>SNAASATETNTAPSADTQAPKPVNTVTSDVDCSVSAAWGLYKFNQKSNFSAEFEMPESVKAGTGFDALIKIKDISVSNDNLSGYKNAKLTKSSIRINVGKNVKLDGNQPGLSLSNGVLSINDHLKASLEGNSLRISAAPITVRLQALTEGTLTFIPEKTILTNTASVDGYTANTTCTTNADKPFATVKVDPADGLTITAPESASIKQDVQITATVPEKLNEKMDGKVQFFVNHIAAGDPVPVTEDNKASTSIIFDTSGSKTITAR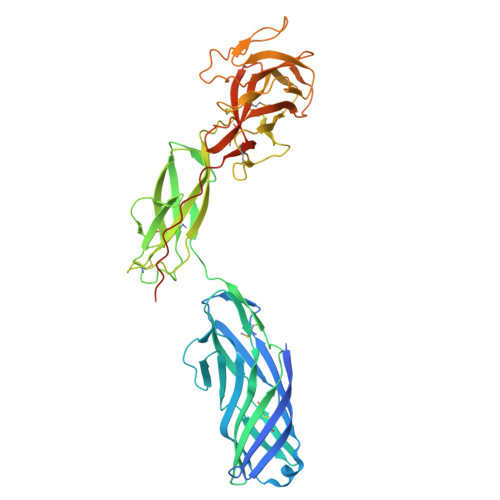FIDAEGYNPAPDGETIIPVVTELDTKKPEDTDSYTGLINGSATSLLKPAKVMPGEKVSVSASLLPNKAPIRVYEIGINAPEDVKYIDGTGKTNYSSKLATTGSVFSSPGSGYYDPEWKNESKKPNESYRGFHSDTSYSVVDTSPQTVSAEFEIPKTLAPGIYMFQMGVYKYSNSLKDLVSIPETAFEIAGPDLPALPERKIKPQPEETPEVSDGSSTAKLVKSP[2x]>[2x]MLIFDDKNYKVDTCNIDGISIKFRSFKEILYCEKPVDSIQKMNIFVPEVYYEGNTINGYSLHTAPIFMPNTVGGYMPGPADEPGKDFKGRINSIFRALKHGYIVVSAGVRGRTSGVKTNE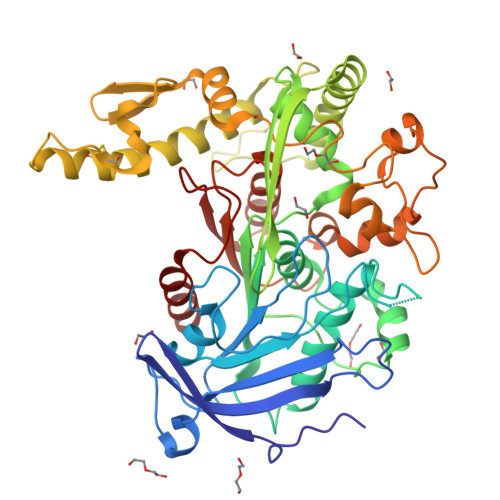FFVGSKAGEISNENGKMVGRAPALVVDMKAAIRYLRYNKGRIPGNTECIVTNGTSAGGALSAIIGASGNSEDYNPYLKEIGAADERDDIFAASCYCPIHNLENADAAYEWQFCGYNDYHRIKHVRSESGVKNIQIDGILTEKQIKISEELKRLFPKYLNSLKLKDSSNNELLLDENGEGSFKEYIKKLVINSAQKELDLCSTYKIIDNAAVCGSKIDEQEYLSIEDEKVVDINWDGFIKKITRMKVAPAFDALDLKSPENEEFGTEAIKAKHFTAYSQEHSEVEGTLADPKIIKLLNPIEYINNSDTAKYWRVRHGAFDRDISLAMPSILSLTLENNGYVVDFSLPWGIPHSGDYDLDDLFAWIDEIYTK PEAK pseudokinases regulate cell migration, invasion and proliferation by recruiting key signaling proteins to the cytoskeleton. PEAK proteins are a unique group of pseudokinase (PsK) scaffolds that can self-assemble regulatory networks. In addition to the conserved PsK and SHED domains, all PEAK proteins have an N-terminal intrinsically disordered region (IDR) replete with short linear motifs (SLiMs)—conserved sequence motifs that can that form dynamically regulated docking sites to recruit interactors involved in PEAK signaling. Here, we elucidate the molecular details of key PEAK signaling interactions with the adapter proteins CrkII and Grb2 and the scaffold protein 14-3-3.

The first was a tyrosine/SH2 motif (YSNL; PEAK3Y24/PEAK1Y1107) that is highly conserved in PEAK3 and PEAK1 vertebrate orthologs (and absent in PEAK2 vertebrate orthologs) that matches the known phosphotyrosine consensus motif for the Grb2 SH2 domain (Grb2SH2; consensus motif: pYxNx) and the CrkII SH2 domain (CrkIISH2; consensus motif: pYxx(P/L), proline typically preferred). We confirm that active Src, but not Abl, phosphorylates the conserved TYSNL SH2-motif (PEAK3Y24, PEAK1Y1107), supporting previous cellular studies, and thereby provides a binding site on either PEAK3 or PEAK1 for Grb2SH2 or possibly CrkIISH2. To do this we utilized a synthetic 7-mer pY phospho-peptide encompassing this SH2 motif (TpYSNLGQ; corresponding to PEAK323–29-pY24 and PEAK11106–1112-pY1107), hereafter “SH2-pY peptide”. We have previously shown by isothermal titration calorimetry (ITC) that this SH2-pY peptide binds to both full length Grb2 (Grb2FL, KD 2.6 µM) and CrkII (CrkIIFL, KD 7.8 µM). Using an approach developed for apo-Grb2FL 36, we succeeded in crystallizing a complex of human Grb2FL:PEAK SH2-pY peptide and solved an X-ray structure to a resolution of 2.7 Å. Close crystal packing within the asymmetric unit leaves only this SH2 site (chain B) available for phosphopeptide binding. Whilst no density was apparent for the C-terminal (-GQ) residues of the peptide, we noticed a potential surface groove directly adjacent on Grb2SH2. In contrast, for Grb2, significant binding to PEAKs is only observed following Src phosphorylation (and only for PEAK3FL and PEAK1IDR1), confirming that direct Grb2 recruitment to PEAKs is primarily SH2-mediated and likely occurring via the consensus pY-SH2 motif we have identified and characterised.

>GSMEAIAKYDFKATADDELSFKRGDILKVLNEECDQNWYKAELNGKDGFIPKNYIEMKPHPWFFGKIPRAKAEEMLSKQRHDGAFLIRESESAPGDFSLSVKFGNDVQHFKVLRDGAGKYFLWVVKFNSLNELVDYHRSTSVSRNQQIFLRDIEQVPQQPTYVQALFDFDPQEDGELGFRRGDFIHVMDNSDPNWWKGACHGQTGMFPRNYVTPVNRNV[2x];> TYSNLGQ>[2x]SLIPEIDAFLGCPTPDAWIEAALADQETLLIDHKNCEFKAASTALSLIAKYNTHLDLINMMSRLAREELVHHEQVLRLMKRRG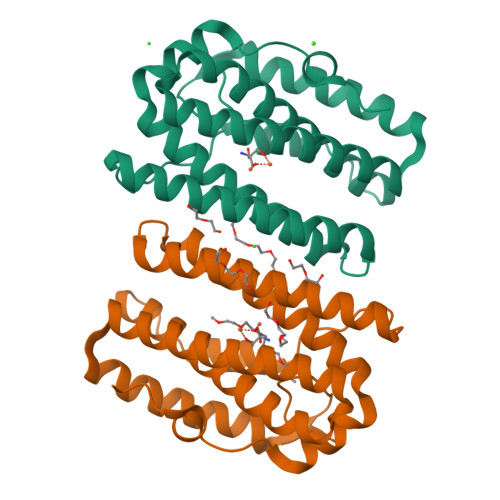VPLRPVSAGRYASGLRRLVRAHEPVKLVDTLVVGAFIEARSCERFAALVPHLDEELGRFYHGLLKSEARHYQGYLKLAHNYGDEADIARRVELVRAAEMELIQSPDQELRFHSGIPQ>GALTTSTRQGSRVVGFMDFIIALGWQIIPSNIRYIYILNCSQFMPTSDVTTIYFQADSGLESI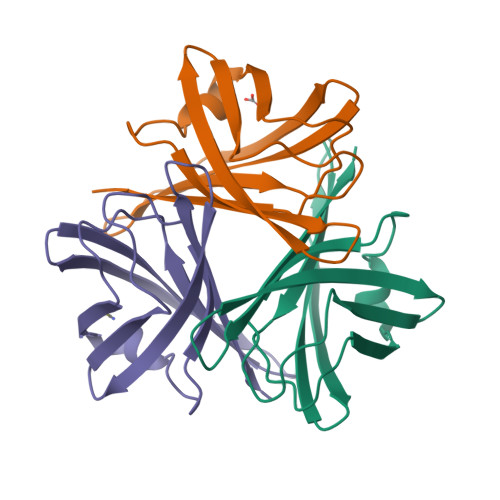FVMDSPFYASCTQQLPDKTIKTYGVTISKKQSIISINFSSSLEPNIMVSAWTASITRTQ[3x]(2R)-N-{3-[(5-fluoro-4-oxopentyl)amino]-3-oxopropyl}-2,4-dihydroxy-3,3-dimethylbutanamide | C14 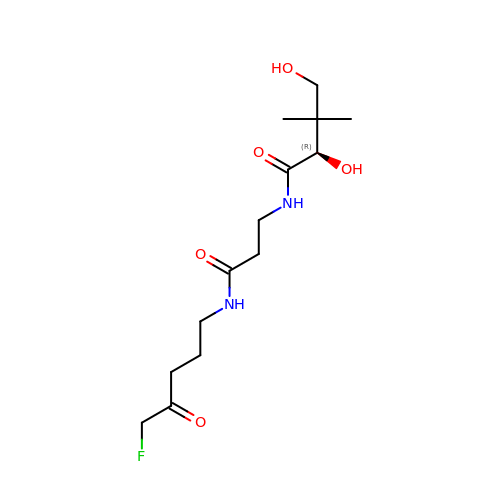H25 F N2 O5 | FTHCNOQGZZPFFG-LBPRGKRZSA-N> SQETFSDLWKL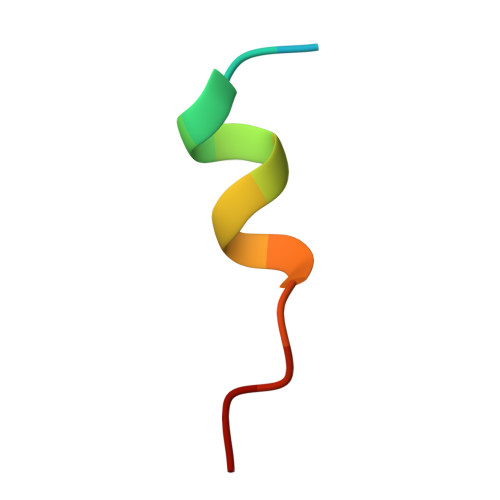LPEN> ASSENASSAKLSVPERQKLAQQSAGKVLTLLDLSEVQLDGAATLVLTFSIPLDPDQDFSRVIHVVDKKSGKVDGAWELSDNLKELRLRHLEPKRDLIVTIGKEVKALNNATFSKDYEKTITTRDIQPSVGFASRGSLLPGKVVEGL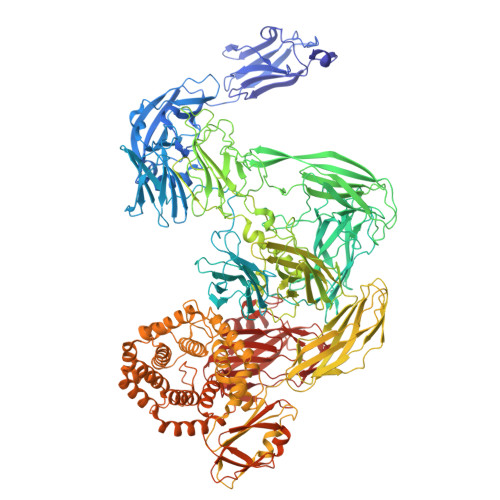PVMALNVNNVDVNFFRVKPESLPAFISQWEYRNSLANWQSDKLLQMADLVYTGRFDLNPARNTREKLLLPLGDIKPLQQAGVYLAVMNQAGRYDYSNPATLFTLSDIGVSAHRYHNRLDIFTQSLENGAAQQGIEVSLLNEKGQTLTQATSDAQGHVQLENDKNAALLLARKDGQTTLLDLKLPALDLAEFNIAGAPGYSKQFFMFGPRDLYRPGETVILNGLLRDADGKALPNQPIKLDVIKPDGQVLRSVVSQPENGLYHFTWPLDSNAATGMWHIRANTGDNQYRMWDFHVEDFMPERMALNLTGEKTPLTPKDEVKFSVVGYYLYGAPANGNTLQGQLFLRPLREAVSALPGFEFGDIAAENLSRTLDEVQLTLDDKGRGEVSTESQWKETHSPLQVIFQGSLLESGGRPVTRRAEQAIWPADALPGIRPQFASKSVYDYRTDSTVKQPIVDEGSNAAFDIVYSDAQGVKKAVSGLQVRLIRERRDYYWNWSEDEGWQSQFDQKDLIENEQTLDLKADETGKVSFPVEWGAYRLEVKAPNEAVSSVRFWAGYSWQDNSDGSGAVRPDRVTLKLDKASYRPGDTIKLHIAAPTAGKGYAMVESSEGPLWWQEIDVRAQGLDLTIPVDKTWNRHDLYLSTLVVRPGDKSRSATPKRAVGVLHLPLGDENRRLDLALETPAKMRPNQPLTVKIKASTKNGEKPKQVNVLVSAVDSGVLNITDYVTPDPWQAFFGQKRYGADIYDIYGQVIEGQGRLAALRFGGDGDELKRGGKPPVNHVNIVVQQALPVTLNEQGEGSVTLPIGDFNGELRVMAQAWTADDFGSNESKVIVAAPVIAELNMPRFMASGDTSRLTLDITNLTDKPQKLNVALTASGLLELVSDSPAAVELAPGVRTTLFIPVRALPGYGDGEIQATISGLALPGETVADQHKQWKIGVRPAFPAQTVNYGTALQPGETWAIPADGLQNFSPVTLEGQLLLSGKPPLNIARYIKELKAYPYGCLEQTASGLFPSLYTNAAQLQALGIKGDSDEKRRASVDIGISRLLQMQRDNGGFALWDKNGDEEYWLTAYVMDFLVRAGEQGYSVPTDAINRGNERLLRYLQDPGMMSIPYADNLKASKFAVQSYAALVLARQQKAPLGALREIWEHRADAASGLPLLQLGVALKTMGDATRGEEAIALALKTPRNSDERIWLGDYGSSLRDNALMLSLLEENKLLPDEQYTLLNTLSQQAFGERWLSTQESNALFLAARTIQDLPGKWQAQTSFSAEQLTGEKAQNSNLNSDQLVTLQVSNSGDQPLWLRMDASGYPQSAPLPANNVLQIERHILGTDGKSKSLDSLRSGDLVLVWLQVKASNSVPDALVVDLLPAGLELENQNLANGSASLEQSGGEVQNLLNQMQQASIKHIEFRDDRFVAAVAVDEYQPVTLVYLARAVTPGTYQVPQPMVESMYVPQWRATGAAEDLLIVRP> MGERPPPKRLTREAMRNYL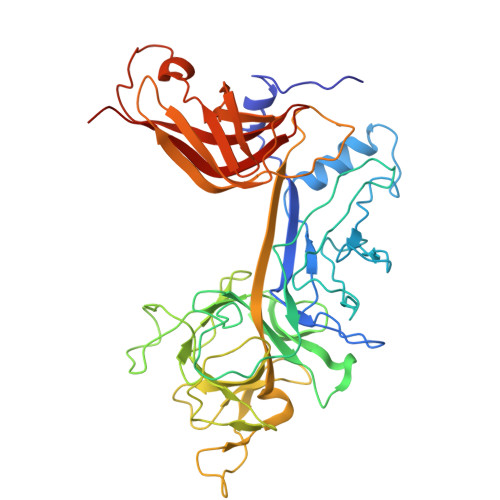KERGDQTVLILHAKVAQKSYGNEKRFFCPPPCVYLMGSGWKKKKEQMERDGCSEQESQPCAFIGIGNSDQEMQQLNLEGKNYCTAKTLYISDSDKRKHFMLSVKMFYGNSDDIGVFLSKRIKVISKPSKKKQSLKNADLCIASGTKVALFNRLRSQTVSTRYLHVEGGNFHASSQQWGAFFIHLLDDDESEGEEFTVRDGYIHYGQTVKLVCSVTGMALPRLIIRKVDKQTALLDADDPVSQLHKCAFYLKDTERMYLCLSQERIIQFQATPCPKEPNKEMINDGASWTIISTDKAEYTFYEGMGPVLAPVTPVPVVESLQLNGGGDVAMLELTGQNFTPNLRVWFGDVEAETMYRCGESMLCVVPDISAFREGWRWVRQPVQVPVTLVRNDGIIYSTSLTFTYTPEPHHHHHH L-METHIONINE-S-SULFOXIMINE PHOSPHATE | C5 H13 N2 O6 P S | 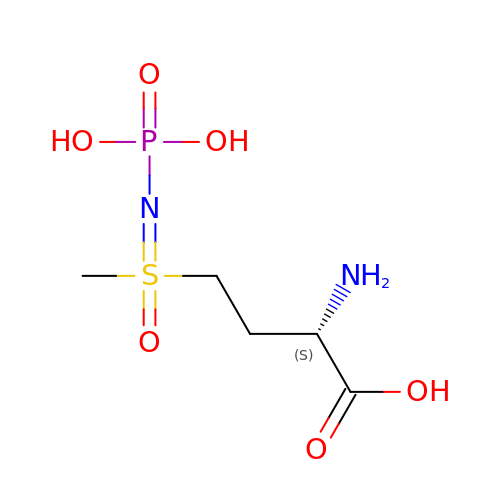QQFOFBSCSWFFPB-NMAPHRJESA-N>[2x]ACDYTCGSNCYSSSDVSTAQAAGYKLHEDGETVGSNSYPHKYNN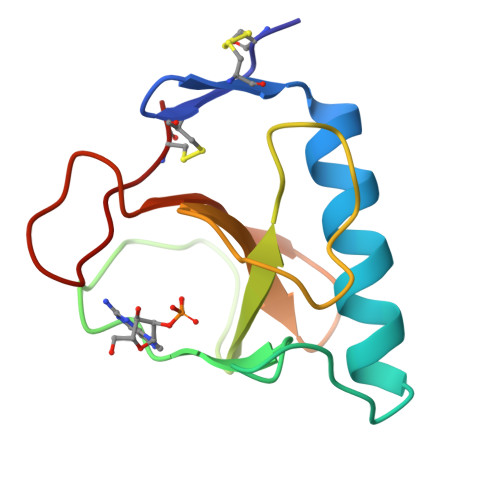YEGFDFSVSSPYYEWPILSSGDVYSGGSPGADRVVFNENNQLAGVITQTGASGNNFVECT>GRKKIQITRIMDERNRQVTFTKRKFGLMKKAYELSVLCDCEIALIIFNSSNKLFQYASTDMDKVLLKYT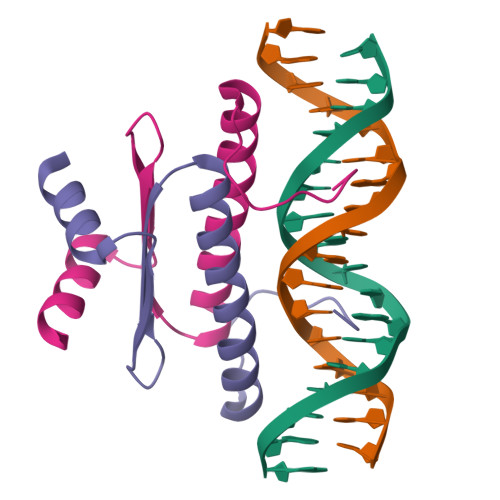EYNEPHES[4x]Glycoside hydrolase family 71 (GH71) includes α-1,3-glucan degrading enzymes which could be exploited for biotechnological applications; however, the family is presently poorly understood. To increase our understanding of GH71, we have performed a phylogenetic analysis of the family and detailed biochemical analysis of two of the five GH71 enzymes encoded by Aspergillus nidulans (AnGH71B and -C). We present the first structure of a GH71 protein, AnGH71C, including structures with carbohydrate ligands. These structures revealed a conserved acidic dyad (DxxE), found to be crucial for activity, and active site water coordination consistent with a classical inverting GH mechanism.

Complexes of AnGH71C with glucose and nigerotriose/nigerotetraose were obtained by soaking crystals with ligand and clearly revealed the binding cleft within the N-terminal (β/α)8-barrel domain. The two protein molecules of the glucose-soaked crystals each contain two glucose molecules located in the same position in the binding cleft, while each of the four protein molecules of the nigerotetraose-soaked crystals contain distinct combinations of nigerotriose and nigerotetraose occupying different subsites within the cleft. Crystals of the apo protein and glucose-soaked crystals were of the C121 space group with similar unit cell dimensions and contained 2 molecules in the asymmetric unit, while the nigerotetraose soak was determined in P1 containing 4 molecules in the asymmetric unit. Only small protein structural changes are observed upon ligand binding in AnGH71C with the most significant being the packing of the loop between β6 and α6 over the substrate along the +1 to +3 sites leading to interactions with Gly193 and Asn194.

>[2x]MGSSHHHHHHSSENLYFQGHSLPGANSLTIRKDSNKYVTAHFMVGIVENYTVDDWKHDMELAKETGIDAFALNCASIDSYTDKQLAYAYEAAEEVDFKVFISFDFAYWSNGDTARITSIMQTYADHPGQFQYNGAALVSTFVGDSFDWGPVKRAVDHPIFAVPNLQDPNWAGHATTSIDGAFSWYAWPTDGGNSIIKGPMTTIWDDRFRNNLKDKVYMAPVSPWFSTHFNTKNWVFICEDLPHLRWQQMLEMQPELIEIISWNDYGESHYIGPYSEAHSDDGSAQWTKDFPHDAWRIIAKPYIAAYKAGEREPTVESDQLVYWYRPTPKAVTCSKDPLGPPNGINLLEDSVFVTTLLTEPATLTVGSGSLEFSVDVDAGIVTNSFPMGVGSQAFSVTRDGEEILGGDGGLDVQDRCDYYNFNVYVGSFSA>MNHKVHHHHHHIEGRHMNEFARAKRALEHSRRINAGDLDAIIDLYAPDAVLEDPVGLPPVTGHDALRAHYEPLLAAHLREEAAEPVAGQDATHALIQISSVMDYLPVGPLYAERGWLKAPDAPGTARIHRTAMLVIRMDASGLIRHLKSYWGTSDLTV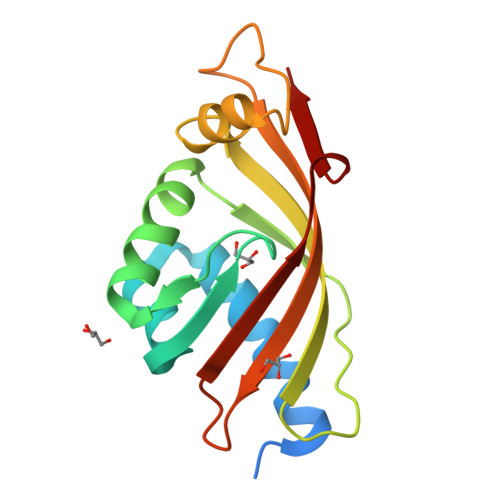LG[2x]> TMITHHHHHHGSMHYKAQLQKLLTTEEKKILARLSTPQKIQDFLDTIKNKDLAEGEHTMWSPRAVLKHKHAHCMEGAMLAALALAYHGHSPLLMDLQTTDEDEDHVVALFKIDGHWGAISKTNHPVLR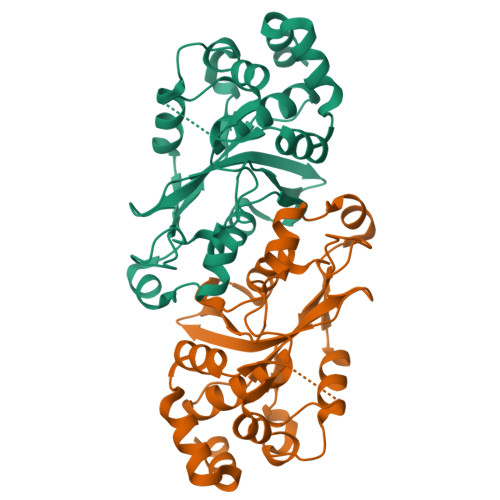YRDPIYKSVRELAMSYFHEYFIWWTKKNGGKKTLRAYSNPFDLTRYKPERWVIATGDLDWLAEALDDSKHFPILNKKMQKQLRPASRIETKAASLSEWPKRKTNS>[2x]GSH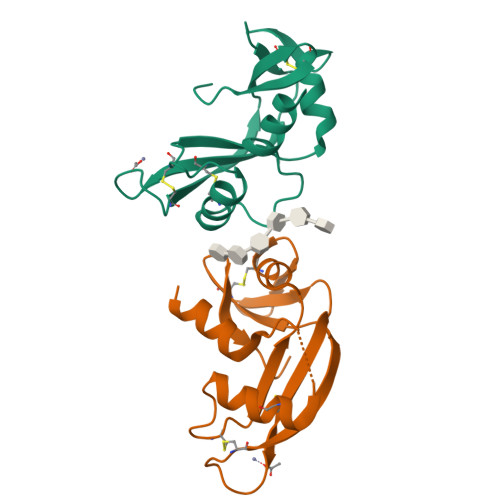MAQDDPRYTKFLTQHYDAKPKGRDARYCESMMRRRGLTSPCKEVNTFIHGNKGSIKAICGANGSPYGENLRISQSPFQITTCKHTGGSPRPPCRYRASAGFRHVVIACENGLPVHFDESFISL> MDLIQAAYFVVAILFIVGLKRMAHPTTAKSGIVWAGWGMVLAVLATFFWPGMGNFALILLALLLGSVVAWWAAVRVAMTDMPQMVAIYNGMGGGAAATIAAVELLKGAFENTGLMALAILGGLIGSVAFTGSLIAFAKLQGIMKSRPILFPGQKAVNALVLALTVVIGLSLLWNDATASIVLFFLLALLFGVLMTLPIGGGDMPVAISFYNAFTGMAVGFEGFAVGNPALMVAGTL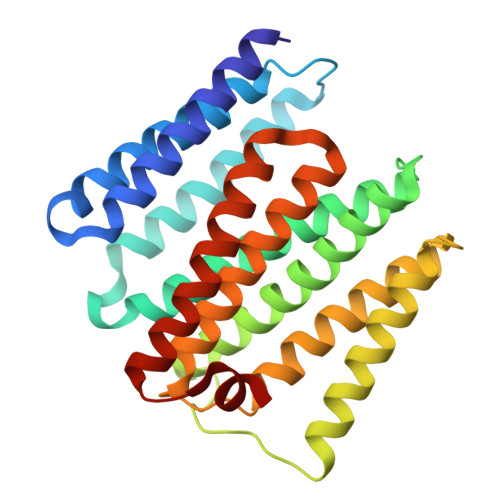VGAAGTLLTVLMARAMNRSVWISVLVGG> AIATYNSHVELAKYLVSKADSVYLTIGKSTPWSNETNPPQPDENATVLQEVIGYKKATKVTLVRPSKSPEDDNKNLISYGNKSW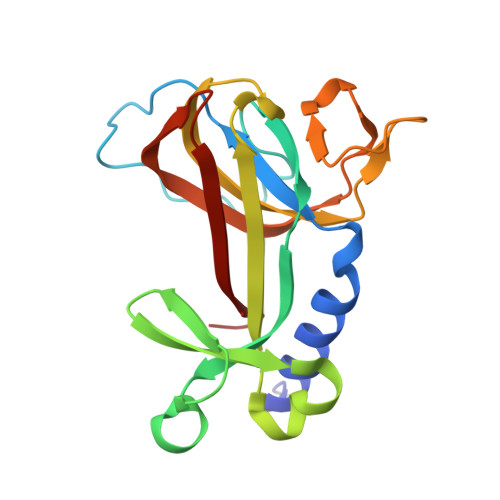VEVTPENAKAEGAKWVYLESSIVGDELPLGTYRQVGFVMDLVAKSGISKFNLVPSEVESTGTLLFFDNKQFQNRSEQTTAKERFIVEVDP> MNKHTNLVTSSFNLTKPMKSFIRRNGLRVQESVTDETDFVILGSPPLRRTHKFLLATSL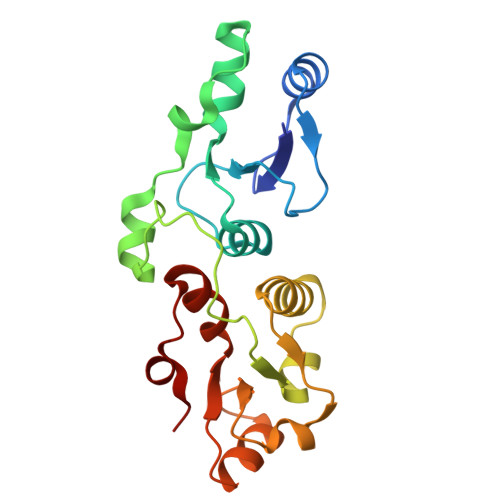GIPLVSSQYLTDCIKSGKVLDFRSYKYKDEEAEAKWGFRLDDIHRRTCFNGKRLYITKAIRDSMVGDSIHGLYSILETSGAEIVGDIKRAQEKDTIILAQPDNDQEGRNMSATGLNVYKIELVALSILRDRIDFDEFLID>[4x]AIA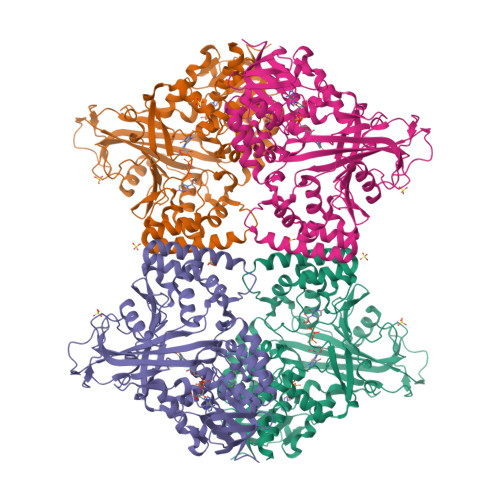MTHPDISVDVLVIGAGPTGLGAAKRLNQIDGPSWMIVDSNETPGGLASTDVTPEGFLYDVGGAVIFSHYKYFDDCLDEALPKEDDWYTHQRISYVRCQGQWVPYPFQNNISMLPKEEQVKCIDGMIDAALEARVANTKPKTFDEWIVRMMGTGIADLFMRPYNFKVWAVPTTKMQCAWLGERVAAPNLKAVTTNVILGKTAGNWGPNATFRFPARGGTGGIWIAVANTLPKEKTRFGEKGKVTKVNANNKTVTLQDGTTIGYKKLVSTMAVDFLAEAMNDQELVGLTKQLFYSSTHVIGVGVRGSRPERIGDKCWLYFPEDNCPFYRATIFSNYSPYNQPEASAALPTMQLADGSRPQSTEAKEGPYWSIMLEVSESSMKPVNQETILADCIQGLVNTEMLKPTDEIVSTYHRRFDHGYPTPTLEREGTLTQILPKLQDKDIWSRGRFGSWRYEVGNQDHSFMLGVEAVDNIVNGAVELTLNYPDFVNGRQNTERRLVDGAQVFAKSKAQ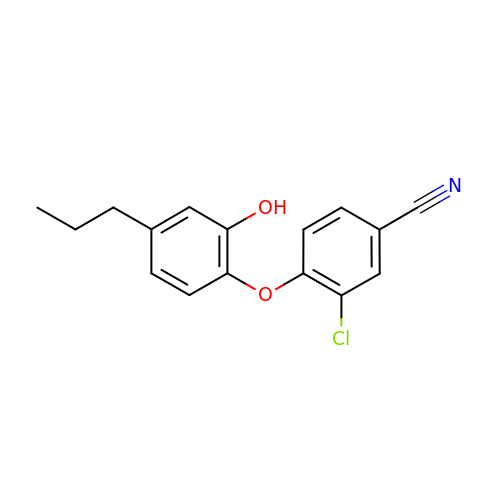3-chloro-4-(2-hydroxy-4-propylphenoxy)benzonitrile | C16 H14 Cl N O2 | KUCPXASBGVCWFQ-UHFFFAOYSA-N>SNGQENGSMFSLITWNIDGLDLNNLSERARGVCSYLALYSPDVIFLQEVIPPYYSYLKKRSSNYEIITGHEEGYFTAIMLKKSRVKLKSQEIIPFPSTKMMRNLLCVHVNVSGNELCLMTSHLESTRG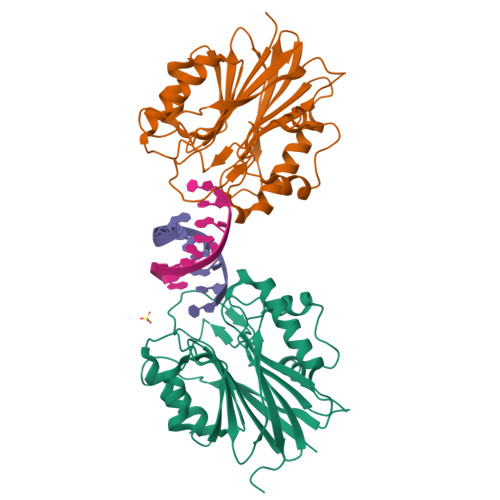HAAERMNQLKMVLKKMQEAPESATVIFAGDTNLRDREVTRCGGLPNNIVDVWEFLGKPKHCQYTWDTQMNSNLGITAACKLRFDRIFFRAAAEEGHIIPRSLDLLGLEKLDCGRFPSDHWGLLCNLDIIL[2x]> SAEKLFTPLKVGAVTAPNRVFMAPLTRLRSIEPGDIPTPLMGEYYRQRASAGLIISEATQISAQAKGYAGAPGLHSPEQIAAWKKITAGVHAEDGRIAVQLWHTGRISHSSIQPGGQAPVSASALNANTRTSLRDENGNAIRVDTTTPRALELDEIPGIVND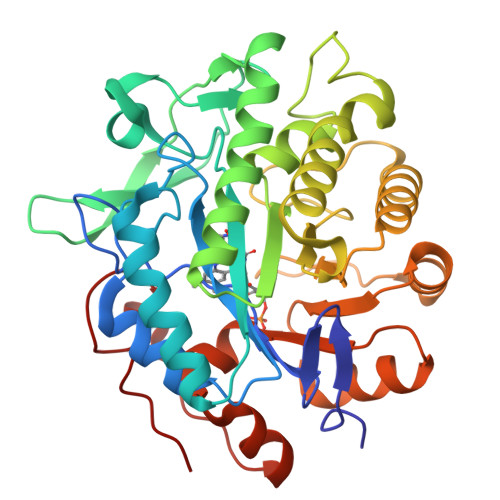FRQAVANAREAGFDLVELHSAHGYLLHQFLSPSSNQRTDQYGGSVENRARLVLEVVDAVCNEWSADRIGIRVSPIGTFQNVDNGPNEEADALYLIEELAKRGIAYLHMSETDLAGGKPYSEAFRQKVRERFHGVIIGAGAYTAEKAEDLIGKGLIDAVAFGRDYIANPDLVARLQKKAELNPQRPESFYGGGAEGYTDYPSL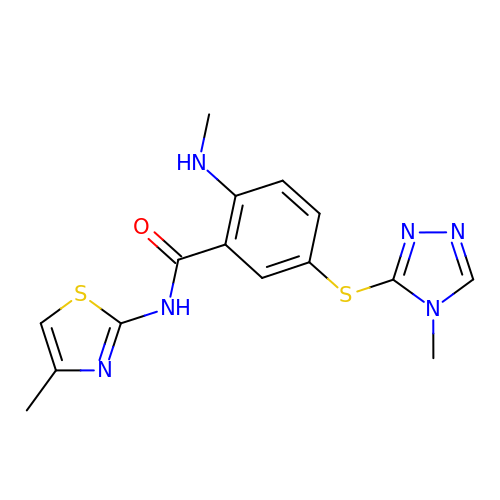2-(methylamino)-N-(4-methyl-1,3-thiazol-2-yl)-5-[(4-methyl-4H-1,2,4-triazol-3-yl)sulfanyl]benzamide | C15 H16 N6 O S2 | XRJAKERBMMBUGR-UHFFFAOYSA-N>[5x]APADNAADARPVDVSVSIFINKIYGVNTLEQTYKVDGYIVAQWTGKPRKTPGDKPLIVENTQIERWINNGLWVPALEFINVVGSPDTGNKRLMLFPDGR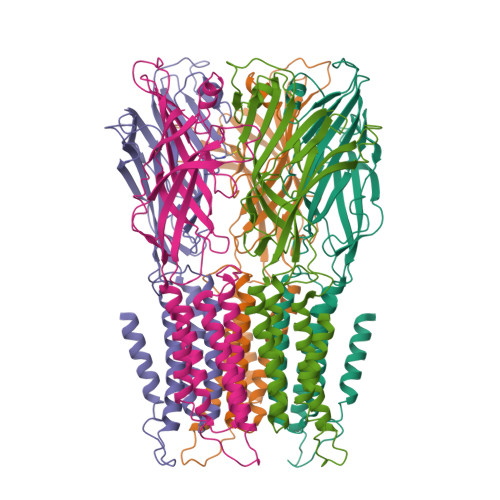VIYNARFLGSFSNDMDFRLFPFDRQQFVLELEPFSYNNQQLRFSDIQVYTENIDNEEIDEWWIRGKASTHISDIRYDHLSSVQPNQNEFSRITVRIDAVRNPSYYLWSFILPLGLIIAASWSVFWLESFSERLQTSFTLMLTVVAYAFYTSNILPRLPYTTYIDQMIIAGYGSIFAAILLIIFAHHRQANGVEDDLLIQRCRLAFPLGFLAIGCVLVIRFFTL> MALEEIRPKEVYLDRKLLTLEDKELGSGNFGTVKKGYYQMKKVVKTVAVKILKNEANDPALKDELLAEANVMQQLDNPYIVRMIGICEAESWMLVMEMAELGPLNKYLQQNRHVTDKNIIELVHQVSMGMKYLEESNFVHRD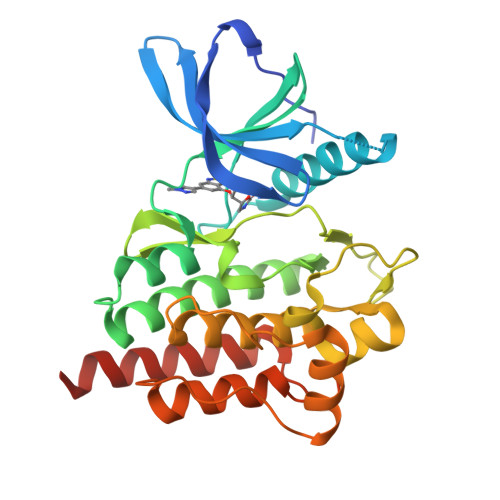LAARNVLLVTQHYAKISDFGLSKALRADENYYKAQTHGKWPVKWYAPECINYYKFSSKSDVWSFGVLMWEAFSYGQKPYRGMKGSEVTAMLEKGERMGCPAGCPREMYDLMNLCWTYDVENRPGFAAVELRLRNYYYDVVNEGHHHHHH> MN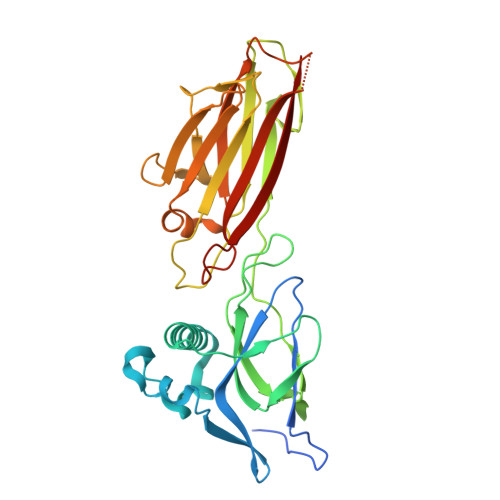HKVHHHHHHIEGRHMTPSISKDAPIKGSITISKKGATFTAYKLLDAIKSGDAYEYSVNSDLKDFFNNSNYGSYSQESIQKLNGEQVKEFAINLHKYILENKKSGQELKDGQKNTVDLGYYLVTETSSDSEGAAVASTPIIVSVPQVSGDSWNYDVTINPKDNTPILEKNIVKENQRVKTSSENIGDVVKYEVKASIPVYQKNAQNIMYKFTDTMSKGLTYDEKTGFKVTSGDKVFAKDTDYTVDVKKQEDGSTVITINFVYENIKAYAETGITLNYQATLNKDAVISNKENLGNTNNIQLDYTNNPHVKDSYKKLTDKVTTYT The Maf polymorphic toxin system is involved in conflict between strains found in pathogenic Neisseria species such as Neisseria meningitidis and Neisseria gonorrhoeae. In the MGIs, the MafB and MafI encode toxin and immunity proteins, respectively. Since MafB contains a specific domain (MafB-CT) in the C-terminal region that has toxic activity, a gene encoding an immunity protein, MafI, is necessary to protect MafB-producing cells from the toxic activity. MafB2MGI-2B16B6 is a polymorphic toxin present in MGI-2 in N. meningitidis strain B16B6 and it has been shown that MafB2-CTMGI-2B16B6 has toxic activity.

In order to infer the enzymatic properties contributing the toxic activity of MafB2MGI-2B16B6, which is the second MafB protein encoded in maf genomic island 2 (MGI-2) from N. meningitidis B16B6, the X-ray crystal structure of the complex between the toxin domain of MafB2MGI-2B16B6, hereafter referred to as NmMafB2-CT, and the corresponding immunity protein, MafI2MGI-2B16B6, hereafter referred to as NmMafI2, was determined at 1.5 Å resolution with 18.0% Rwork and 20.8% Rfree using a single anomalous dispersion method. However, the N-terminal 53 residues from Ala270 to Ser322 of NmMafB2-CT were invisible probably due to the degradation of NmMafB2-CT during crystallization. The overall structure of NmMafB2-CT2 has a kidney-like shape characterized by an RNase A fold and consists of two central β-sheets with three peripheral α-helices. The structure of NmMafI2 consists of a four-stranded central β-sheet, one strand (β4′) of which is relatively short, and three helices. In the structure of the NmMafB2-CT2/NmMafI2 complex, the α2′ helix flanked by α1′ of NmMafI2 packs tightly against the shallow groove of NmMafB2-CT2. The interaction between NmMafB2-CT2 and NmMafI2 is mediated by extensive hydrophobic and hydrogen bond interactions including eight salt bridges. Notably, the residues in α2′ of NmMafI2 contributes approximately 65% of the hydrogen bond and salt bridge interactions. Upon complex formation, approximately 1110 Å2 of the binding interface becomes buried, which corresponds to approximately 17.0% and 17.5% of the surface areas of NmMafB2-CT2 and NmMafI2, respectively. All negatively charged residues of NmMafI2 in the complex interface contribute to salt-bridge interactions with NmMafB2-CT2, except that Glu74 of NmMafI2 forms hydrogen bonds with NmMafB2-CT2. These results indicate that complementary charge interactions are the main driving force for the formation of the complex between NmMafB2-CT2 and NmMafI2, and that NmMafI2 functions as an inhibitory regulator protein by blocking RNA from accessing the enzymatic cleavage site because it binds the substrate binding site of NmMafB2-CT2. The dissociation constant of the NmMafB2-CT2/NmMafI2 complex was measured to be ~ 40 nM.

> MGNILPSWLRVGMNIAMLGMIHSDIRLITVDYEERRRFLKIKNYLSREAITEDHEDMEYLITELWSMCGEYFDEADFECIYSNHSSMELNQINGAVFRRKELISQALE;> GHMAKVKNLTKAAKPGKAAVSGDFSDSYKHNTASRLSQSVDGEMFQTRNVDFKAKSIGTKIHDGAQGKHISGHRNYIEGKSTLNQNINPQELLNGIHSGAYPVISKGARRNPVVDFGYPIGSDGKSGLSTNFGTIHSGKNGVHIVPANPKTIKKVQLE>GMGFLDALMGNASEVDLGKLAAELSPILGDNEELQLAYKMVRDLFVFTSKRLILIDKQGVTGKKVSYHSIPYKAIVHFQVETAGTFDMDAELKLWISGQHEPLVKELKRGTDVVGIQKTIARYALG[5x]

As part of our structural genomics effort in targeting novel protein families, we determined crystal structures of three bacterial proteins from a previously structurally uncharacterized protein family Pfam PF08000 [also known as domain of unknown function family 1696 (DUF1696)],11 which appears to be involved in the bacterial cell envelope stress response. These structures share a common domain that is surprisingly similar to the eukaryotic PH-like domains, thus providing the first direct evidence for the existence of PH-like domains in prokaryotes. PHb1 and PHb2 share a common domain that is structurally similar to eukaryotic PH domains, which we have defined as a PHb domain (PH domain in bacteria). The PHb proteins form oligomeric ring assemblies of different sizes and symmetries, providing an excellent example of how molecular architecture can evolve, where the general form of the molecular assembly is preserved, but its size is expandable.

Structure determination of full-length (sa) was enabled using reductive methylation of the protein prior to crystallization. The two PHb1s are closely related (80% sequence identity); PHb1(sa) can be aligned to PHb1(sl) without gaps except for an extra glycine at its C-terminus. The PHb1(sa) model consists of 585 protein residues, 2 polyethylene glycol (PEG) fragments, 6 glycerols, and 242 waters, and PHb2 has 1106 residues and 173 waters. The N-terminal residues, which were deleted in the PHb1(sl) construct, are ordered in two monomers (A and B) of PHb1(sa) due to crystal contacts and form a short helix (α-1, residues 5–11). The conformation of the N-terminal region differs significantly between PHb1(sa) and PHb1(sl). PHb1(sa) does not contain the first strand (β0) found in PHb1(sl). These structural variations, which likely reflect differences in the contact environments in the crystals, demonstrate the inherent flexibility of the PHb domains. The PHb1(sa) pentamer is similar to that of PHb(sl); thus, we refer only to PHb1(sl) in the discussion hereafter. The PHb domains in two PHb1 orthologs contain a structurally conserved core, except for the N-termini (before α0), the L34 loop, and the L56 loop regions that are highly variable in conformation. The 10 copies of the PHb1 monomers [from the two pentamers of PHb1(sl) and PHb1(sa)] can be superimposed with an average rmsd of 1.31 Å for 94 aligned Cα atoms; the rmsd values between different monomers are significantly higher if all variable regions were included.> MGASGTTGVFYYKTGDMQTDDTNHVRWFLNINNENAYVDSDIRIEDDIQSGQTLDIDSFDITVNGSESYRGQEGINQLAQRYGATISADSASGHISVYIPQGYASLNSFSIMYLTKVDNPDQKTFENNSKAWYKENGKDA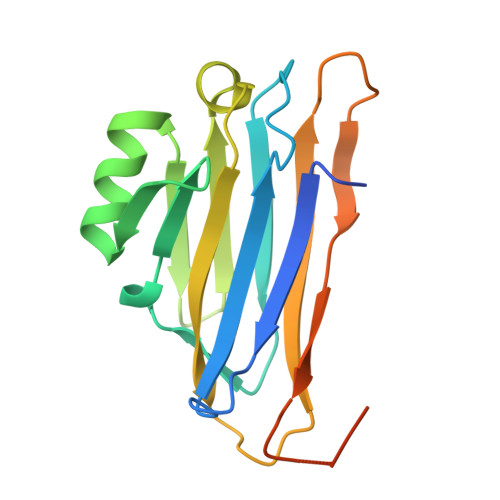VDGKEFNHSVANVNAAGGVDGRENLYFQGLEHHHHHH>[3x]ARSTNTFNYATYHTLDEIYDFMDLLVAEHPQLVSKLQIGRSYEGRPIYVLKFSTGGSNRPAIWIDLGIHSREWITQATGVWFAKKFTEDYGQDPSFTAILDSMDIFLEIVTNPDGFAFTHSQN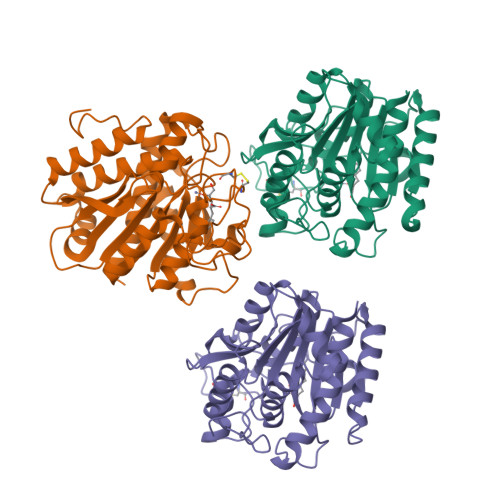RLWRKTRSVTSSSLCVGVDANRNWDAGFGKAGASSSPCSETYHGKYANSEVEVKSIVDFVKDHGNFKAFLSIHSYSQLLLYPYGYTTQSIPDKTELNQVAKSAVEALKSLYGTSYKYGSIITTIYQASGGSIDWSYNQGIKYSFTFELRDTGRYGFLLPASQIIPTAQETWLGVLTIMEHTVNN> MPSEQRGQHRSGYGLGLSTRTQVTGYQFLARRTAMALTRWRVRMEVEPGRRQVLAVVASVSAAGVICLGALLWSFISPSGQMGESPIIADRDSGALYVRVGDTLYPALNLASARLIAGRAENPHKVRSSQIAEQPHGPMVGIPGAPSDISPTSPASSSWLVCDAVTAAQGVGAPASVTVTVIDGTPDLSGRRHVLSGSDAVVLRYGNDTWVIRQGRRSRIDAANRAVLLPLGLTPEQVKQASPMSRALYDALPVGPELAVPKVPDAGKPANFPGAPAPVGAVLVTPQISGP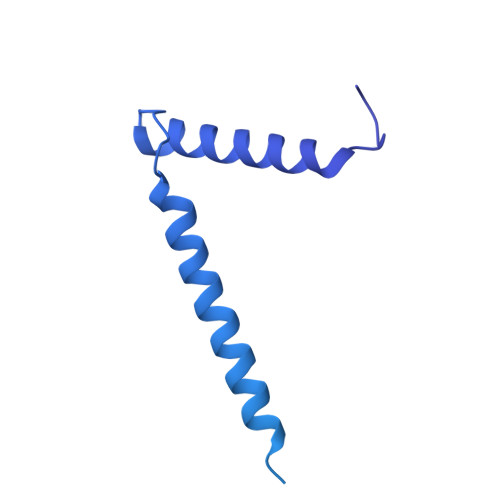QQYSVVLPDGVQTISPIVAQILQNAGTPAGSMPVVVAPATLARMPVVHGLDLSAYPDSPLNVVNMKENPATCWWWEKTAGEERARTQVVSGPTVPIATSDTNKVVSLVKADNTGREADRVYYGPNYANFVVVTGNDPAASTAESLWLLSKSGVRFGVDNSREARTALGLTSTPSPAPWVALRLLAPGPMLSRADALVRHDTLPTDTNPAELAVPK>[4x]GSHMVAAGDNKIKQGLLPSLEDLLFYTIAEGQEKIPVHKFITALKSTGLRTSDPRLKECMDMLRLTLQTTSDGVMLDKDLFKKCVQSNIVLLTQAFRRKFVIPDFMSFTSHIDELYESAKKQSGGKVADYIPQLAKFSPDLWGVSVCTVDGQRHSIGDTKVPFCLQSCVKPLKYAIAVNDL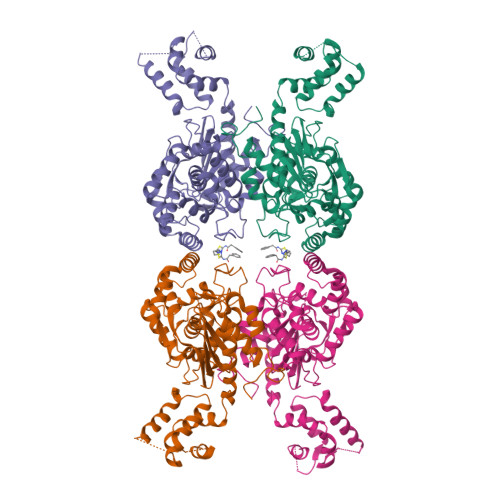GTEYVHRYVGKEPSGLRFNKLFLNEDDKPHNPMVNAGAIVVTSLIKQGVNNAEKFDYVMQFLNKMAGNEYVGFSNATFQSERESGDRNFAIGYYLKEKKCFPEGTDMVGILDFYFQLCSIEVTCESASVMAATLANGGFCPITGERVLSPEAVRNTLSLMHSCGMYDFSGQFAFHVGLPAKSGVAGGILLVVPNVMGMMCWSPPLDKMGNSVKGIHFCHDLVSLCNFHNYDNLRHFAKKLDPRREGGDQRHSFGPLDYESLQQELALKDTVWKKVSPESSDDTSTTVVYRMESLGERS>SHMMASV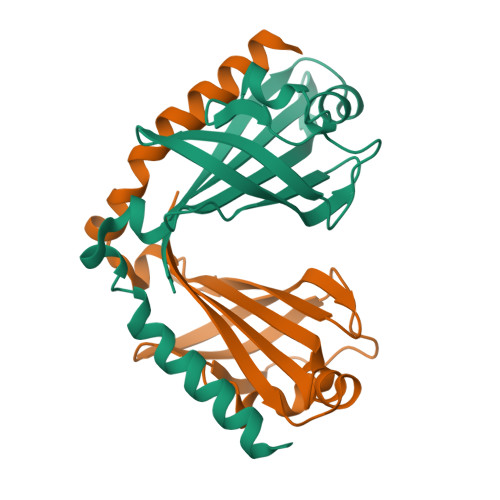ELSADVPISPQDTWDHVSELSELGEWLVIHEGWRSELPDQLGEGVQIVGVARAMGMRNRVTWRVTKWDPPHEVAMTGSGKGGTKYGVTLTVRPTKGGSALGLRLELGGRALFGPLGSAAARAVKGDVEKSLKQFAELYG[4x]>MVGAGAYAYKTMKEDEKRYNERISGLGLTPEQKQKKAALSASEGEEVPQDKAPSHVPFLLIGGGTAAFAAARSIRARDPGARVLIVSEDPELPYMRPPLSKELWFSDDPNVTKTLRFKQANGKERSIYFQPPSFYVSAQDLPHIENGGVAVLTGKKVVQLDVRDNMVKLNDGSQITYEKCLIATGGTPRSLSAIDRAGAEVKSRTTLFRKIGDFRSLEKISREVKSITIIGGGFLGSELACALGRKARALGTEVIQLFPEKGNMGKILPEYLSNWTMEKVRREGVKVMPNAIVQSVGVSSGKLLIKLKDGRKVETDHIVAAVGLEPNVELAKTGGLEIDSDFGGFRVNAELQARSNIWVAGDAACFYDIKLGRRRVEHHDHAVVSGRLAGENMTGAAKPYWHQSMFWSDLGPDVGYEAIGLVDSSLPTVGVFAKATAQDNPKSATEQSGTGIRSESETESEASEITIPPSTPAVPQAPVQGEDYGKGVIFYLRDKVVVGIVLWNIFNRMPIARKIIKDGEQHEDLNEVAKLFNIHEDLEVLFQ[2x]

A 60-kDa FAD-dependent oxidoreductase, AIF allosterically switches between two distinct redox states. NADH binding by the oxidized AIF monomer reduces its FAD cofactor at a centralized active site, allosterically disrupting hydrogen bond networks to release a 50-residue surface loop (C-loop) and stimulate dimerization at the AIF surface. Oxidized NAD+ and reduced FADH– form a long-lived charge-transfer complex (CTC), which stabilizes and maintains the reduced dimeric state of AIF. NADH-activated AIF dimers support import of OXPHOS subunits by CHCHD4 and are critical for mitochondrial function.

To understand how SAXS CX1 and CX2 chemotypes engage AIF and enable dimerization, we crystallized select fragment hits with the W196A dimer-permissive mutant and wild-type AIF. Crystal structures of the W196A mutant bound to CX1 fragments and the underlying 4-aminoquinoline (4AQ) scaffold revealed that these scaffolds localize to the NADH active site, mirroring the native NADH ligand, as do CX1 and CX2 scaffolds bound to the wild-type protein. In all four W196A structures, the CX1 quinoline core aromatically pairs with the AIF FAD cofactor, positioning the primary amine to hydrogen bond with the E314 side-chain carboxylate and the W483 backbone carbonyl. To accommodate this amine interaction, the aromatic side chain of F482 must rotate out of the binding site. Halogen substitutions at positions 7 and 8 (fragments C12, D1 and D3) optimally accelerate dimerization. In addition to hydrogen bonding between the primary amine and AIF active site, the structure of top-ranked fragment C12 additionally reveals a unique halogen-π contact, which places electronegative fluorine compactly against the F482 and H454 aromatic rings, reinforcing their pairing. Although fluorine attraction reverses and rotates the aminoquinoline scaffold, the primary amine still hydrogen bonds with the active site. The dimer-permissive W196A mutant also allosterically releases H454 into the active site, absent NADH ligand binding. This points to H454 release as a preconfiguring event that allows CX1 fragments to engage the AIF active site and stabilize the dimer. When the AIF(W196A) mutant is co-incubated with CX1 fragments, the oxidized mutant fully dimerizes and remains dimeric throughout the time series, similar to the wild-type AIF–NADH–DMSO control.>[2x]DRHHHHHHKLNLTCPACKVLFTALNHGLKKEPNVARVGSVAIKICKMLNIAPLDVCQSAVHLFEDDVVEVWTRSVLSPSEACGLLLGSSCGHWDIFSTWNISLPSVPKPPPKPPSPPAPGAPVSRVLFLTDLHWDHE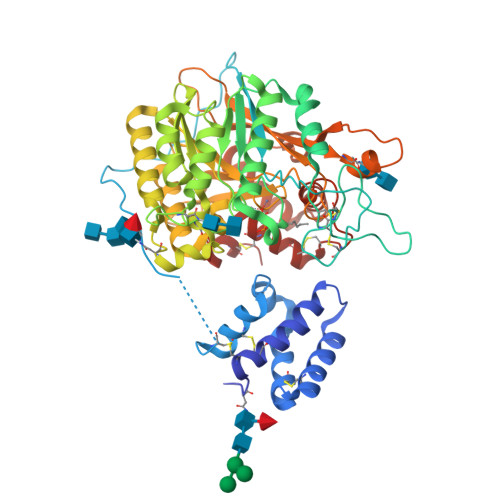YLEGTDPYCADPLCCRRGSGWPPNSQKGAGFWGEYSKCDLPLRTLESLLKGLGPAGPFEMVYWTGDIPAHDVWQQSRQDQLRALTTITDLVRKFLGPVPVYPAVGNHESTPVNGFPPPFIKGNQSSQWLYEAMAKAWEPWLPADALHTLRIGGFYALTPRPGLRLISLNMNFCSRENFWLLINSTDPAGQLQWLVEELQAAENRGDKVHIIGHIPPGHCLKSWSWNYYKIIARYENTLAGQFFGHTHVDEFEIFYDEETLSRPLAVAFLAPSATTFINLNPGYRVYQIDGNYPGSSHVVLDHETYILNLTQANAAGGTPSWKRLYRARETYGLPDAMPASWHNLVYRMRDDEQLFQTFWFLYHKGHPPSEPCGTPCRLATLCAQLSARADSPALCRHLMPN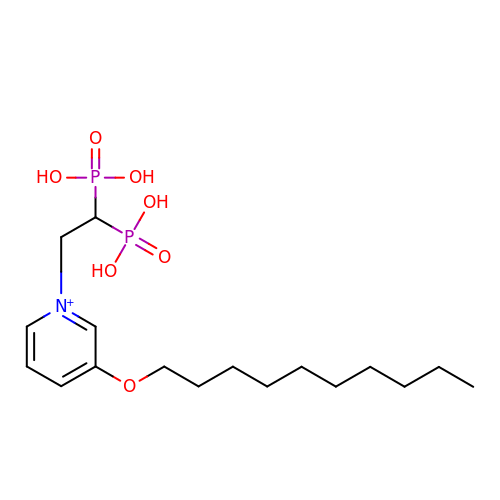3-(DECYLOXY)-1-(2,2-DIPHOSPHONOETHYL)PYRIDINIUM | C17 H32 N O7 P2 | QYJHUOZDBUEKQC-UHFFFAOYSA-O> MELKHSISDYTEAEFLEFVKDIFRLSRPQDNDLQIKLVLEFKRLTEHPDGSDLIYYPRSDREDSPEGIVKEIKEWRAANGKSGFKQGLEHHHHH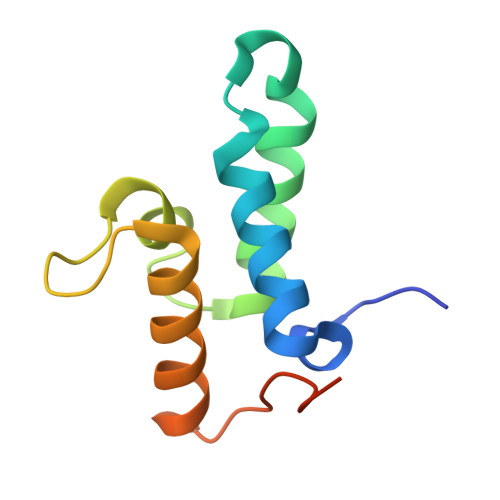H> NLIPTVIEQTNRGERAYDIYSRLLKDRIIMLGSAIDDNVANSIVSQLL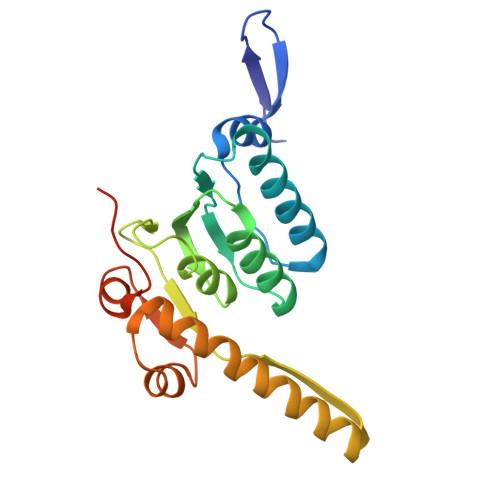FLAAEDPEKEISLYINSPGGSITAGMAIYDTMQFIKPKVSTICIGMAASMGAFLLAAGEKGKRYALPNSEVMIHQPLGGAQGQATEIEIAAKRILLLRDKLNKVLAERTGQPLEVIERDTDRDNFKSAEEALEYGLIDKILTHTEDKKHHHHHH> GSHMATYYYALGSQKFLLEEEPFEEVLKERRRDYGEKNKEIDFWQVIQPAFLNAPELAEAKAKAPEKNVAIVSTNKSFIVWVKLRLEYVLTGEFEAPSDAIPDPLASLD

Mg-protoporphyrin IX monomethylester cyclase (MgPME–cyclase) catalyses the formation of the isocyclic E ring by cyclising the methyl propionate side-chain at C-13 to the C-15 bridge carbon between rings C and D, generating protochlorophyllide (Pchlide). Recently, the small monomeric protein Ycf54 was identified as a second candidate component of the MgPME–cyclase. The Ycf54 protein has been identified as a component of the MgPME–cyclase complex.

A fourth Ycf54 mutant in which residue A9 was substituted with a glycine reduced Ycf54 levels by ∼75% and CycI levels by ∼50%. The FLAG-A9G construct, which like the A9G point mutation was present at lower cellular levels, pulled down CycI in quantities similar to those observed in the FLAG-Ycf54 control pulldown. Therefore, it is reasonable to conclude that although only a small amount of A9G accumulates, there is more than enough Ycf54 protein available to interact with CycI, so allowing the MgPME–cyclase to proceed unhindered. To investigate the structural basis for these effects of the A9G and R82A mutations in Synechocystis, crystal structures solved by molecular replacement against the WT Synechocystis Ycf54 were obtained for these two proteins to resolutions of 1.5 Å and 2.2 Å, respectively. Superposition of the A9G and R82A models on WT Ycf54 resulted in respective RMSDs of 0.19 Å and 0.28 Å over all Cα atoms, showing that there are no significant structural alterations between the WT and mutant structures. Thus, the phenotypes observed in A9G and R82A are not a result of the mutant proteins adopting a different conformation or failing to fold. Further analysis of the local structure around the A9G mutation shows that there are no alterations in the immediate hydrogen bonding network or surface electrostatics, indicating that the phenotypic consequences of the A9G mutation do not result from alterations in the structure. Comparison of the WT and A9G structures found no structural reason for the low levels of A9G observed in vivo. As our pulldown experiments show A9G Ycf54 interacts with CycI at levels comparable to WT Ycf54, it is unlikely that the reduced level of A9G has a structural basis. One explanation for the lower level of A9G could be that the glycine codon inserted is rare in Synechocystis, resulting in lower levels of A9G Ycf54 translation.>MESRYVLTGRYDSAPATDGSGTALGWTVAWKNNYRNAHSATTWSGQYVGGAEARINTQWLLTSGTTEANAWKSTLVGHDTFTKVKPSAASGGGSAEAGITGTWYNQLGSTFIVTAGADGAL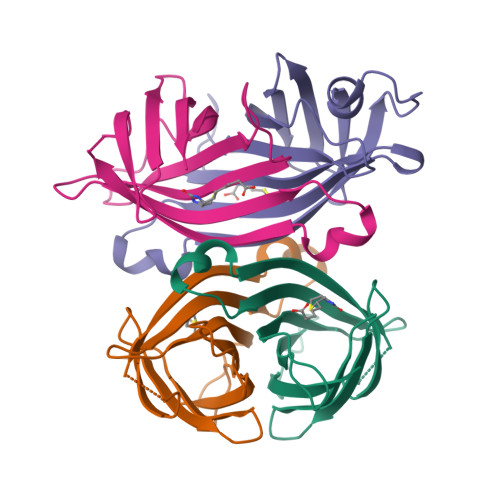TGTYESA[4x]> GAMGSVANVGSHCDLSLKIPEISIQDMTAQVTSPSGKTHEAEIVEGENHTYCIRFVPAEMGTHTVSVKYKGQHVPGSPFQFTVGPLGEGGAHKVRAGGPGLERAEAGVPAEF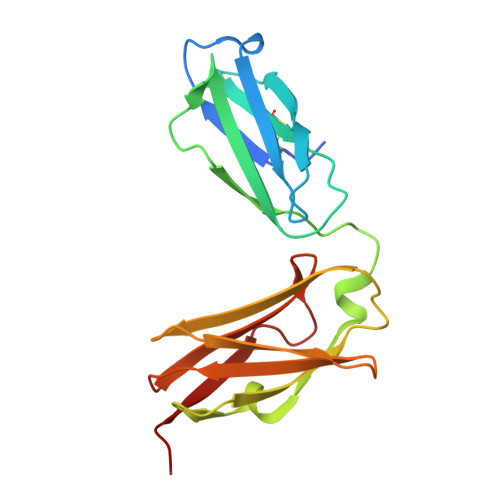SIWTREAGAGGLAIAVEGPSKAEISFEDRKDGSCGVAYVVQEPGDYEVSVKFNEEHIPDSPFVVPVASPS> MHHHHHHAVRASEISRVYEAYPEKKATLYFLVLGFLALIVGSLFGPFQALNYGNVDAYPLLKRLLPFVQSYYQGLTLHGVLNAIVFTQLFAQAIMVYLPARELNMRPNMGLMWLSWWMAFIGLVVAALPLLANEATVLYTFYPPLKGHWAFYLGASVFVLSTWVSIYIVLDLWRRWKAANPGKVTPLVTYMAVVFWLMWFLASLGLVLEAVLFLLPW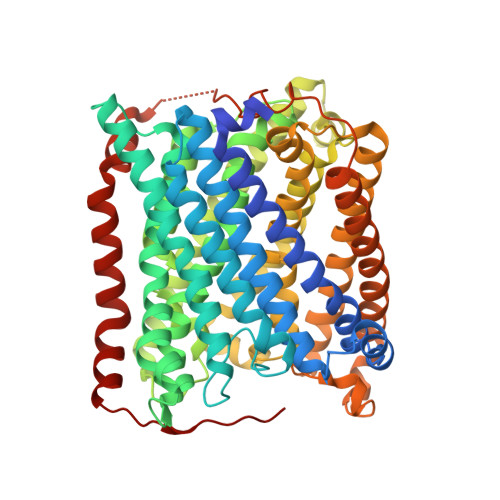SFGLVEGVDPLVARTLFWWTVHPIVYFWLLPAYAIIYTILPKQAGGKLVSDPMARLAFLLFLLLSTPVGFHHQFADPGIDPTWKMIHSVLTLFVAVPSLMTAFTVAASLEFAGRLRGGRGLFGWIRALPWDNPAFVAPVLGLLGFIPGGAGGIVNASFTLDYVVHNTAWVPGHFHLQVASLVTLTAMGSLYWLLPNLTGKPISDAQRRLGLAVVWLWFLGMMIMAVGLHWAGLLNVPRRAYIAQVPDAYPHAAVPMVFNVLAGIVLLVALLLFIYGLFSVLLSRERKPELAEAPLPFAEVISGPEDRRLVLAMDRIGFWFAVAAILVVLAYGPTLVQLFGHLNPVPGWRLW>AVSKVYARSVYDSRGNPTVEVELTTEKGVFRSIVPSGANTGVHEALEMRDGDKSKWMGKGVLHAVKNVNDVIAPAFVKANIDVKDQKAVDDFLISLDGTANKSKLGANAILGVSLAASRAAAAEKNVPLYKHLADLSKSKTSPYVLPVPFLNVLNGGSHAGGALALQEFMIAPTGAKTFAEALRIGSEVYHNLKSLTKKRYGASAGNVGDEGGVAPNIQTAEEALDLIVDAIKAAGHDGKIKIGLDCASSEFFKDGKYDLDFKNPNSDKSKWLTGPQLADLYHSLMKRYPIVSIEDPFAEDDWEAWSHFFKTAGIQIVADALTVTNPKRIATAIEKKAADALLLK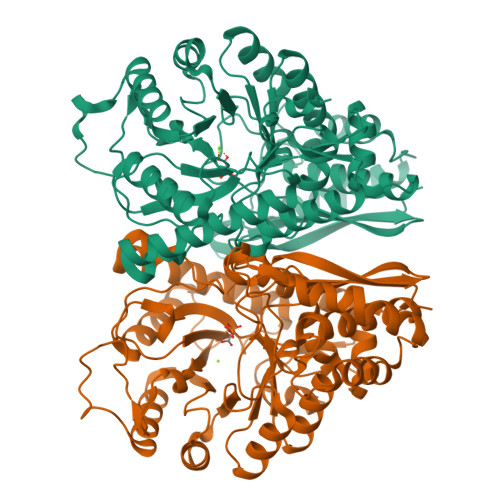VNQIGTLSESIKAAQDSFAAGWGVMVSHRSGETEDTFIADLVVGLRTGQIKTGAPARSERLAKLNQLLRIEEELGDNAVFAGENFHHGDKLLHHHHHH[4x]(1R,5R)-1,5-dihydroxy-4-oxo-3-[3-oxo-3-(phenylamino)propyl]cyclohex-2-ene-1-carboxylic 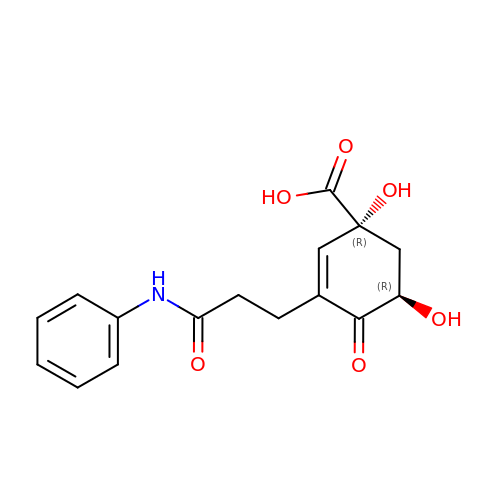acid | C16 H17 N O6 | LCRSMARNUPCDAZ-WBMJQRKESA-N>[4x]GGSEQEIVNLFIPTQAVGAIIGKKGAHIKQLARFAGASIKIAPAEGPDVSE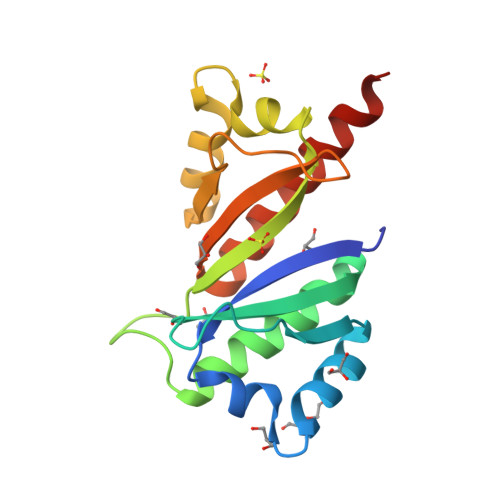RMVIITGPPEAQFKAQGRIFGKLKEENFFNPKEEVKLEAHIRVPSSTAGRVIGKGGKTVNELQNLTSAEVIVPRDQTPDENEEVIVRIIGHFFASQTAQRKIREIVQQVKQQEQK>DPGTIVHNFSRTEPRTEPAGGSHSGSSSKLQALFAHPLYNVPEEPPLLGAEDSLLASQEALRYYRRKVARWNRRHKMYREQMNLTSLDPPLQLRLEASWVQFHLGINRHGLYSRSSPVVSKLLQDMRHFPTISADYSQDEKALLGACDCTQIVKPSGVHLKLVLRFSDFGKAMFKPMRQQRDEETPVDFFYFIDFQRHNAEIAAFHLDRILDFRRVPPTVGRIVNVTKEILEVTKNEILQSVFFVSPASNVCFFAKCPYMCKTEYAVCGKPHLLEGSLSAFLPSLNLAPRLSVPNPWIRSYTLAGKEEWEVNPLYCDTVKQIYPYNNSQRLLNVIDMAIFDFLIGNMDRHHYEMFTKFGDDGFLIHLDNARGFGRHSHDEISILSPLSQCCMIKKKTLLHLQLLAQADYRLSDVMRESLLEDQLSPVLTEPHLLALDRRLQTILRTVEGCIVAHGQQSVIVDGPVEQ[2x];>MILFRKFRVLILTVFLIACTMHIMIDLLPKLEKRAAGSSSSAGGGSGCSCAHTPGEEPRSWGKQRARAADPGWPNKHSLRLLQDFSNEPNSNLTSQSREKVTERAGSEKQGSGKRGLMREADSRQRRTDVRVSSVLQSLFEHPLYRTVLPDLTEEDTLFNLNAEIRLYPKAAGQQEWHNEGNVEEEEFSPPGEANSESYPNWLRFHIGINRYELYSRHNPVIAALLRDLLSQKISSVGMKSGGTQLKLIMSFQNYGQALFKPMKQTREQETPPDFFYFSDFERHNAEIAAFHLDRILDFRRVPPVAGRLVNMTREIRDVTRDKKLWRTFFVSPANNICFYGECSYYCSTEHALCGKPDQIEGSLAAFLPDLALAKRKTWRNPWRRSYHKRKKAEWEVDPDYCDEVKQTPPYDRGTRLLDIMDMTIFDFLMGNMDRHHYETFEKFGNDTFIIHLDNGRGFGKHSHDEMSILVPLTQCCRVKRSTYLRLQLLAKEEYKLSSLMEESLLQDRLVPVLIKPHLEALDRRLRLVLKVLSDCVEKDGFSAVVENDLDGQPSVHGGR[2x]

The Fam20 proteins are recently identified kinases that regulate essential cellular processes by phosphorylating proteins and proteoglycans. The human genome encodes three Fam20 paralogs: Fam20A, Fam20B, and Fam20C13. Remarkably, each has a distinct biochemical activity. Here, we use a combination of structural biology, biochemistry, and phylogenetics to elucidate the molecular functions and evolutionary relationships of the three Fam20 kinases.

In an attempt to address this discrepancy, we solved the structure of the Fam20A−drFam20C complex that is crystallized in a different space group. A four-leaf clover-shaped tetramer is clearly present in this structure, formed by two Fam20A−drFam20C heterodimers similar to the human Fam20A−Fam20C heterodimer shown in Fig. 1a. In light of this Fam20A−drFam20C tetramer structure, we realized that the absence of a human Fam20A−Fam20C tetramer in the crystal is also due to an unexpected obstructing ATP molecule, besides crystal packing effects. Both Fam20A−Fam20C and Fam20A−drFam20C only crystallized in the presence of ATP, likely because ATP significantly stabilizes Fam20A. In both structures, an ATP molecule (ATP-1) is bound to Fam20A in an inverted orientation, as we previously reported. Given that Asn298A is at the center of the Fam20A−drFam20C tetramer interface, the bulky glycan addition is predicted to hinder tetramer formation. Nevertheless, both mutants activated Fam20C at levels comparable to WT Fam20A in vitro and in cells. These data suggest that while a Fam20A−Fam20C heterodimer is required for Fam20A to enhance Fam20C activity, further assembly of a tetramer is dispensable for activation.>MDKDEAWKQVEILRRLGAKRIAYRSDDWRDLQEALKKGADILIVDATDKDEAWKQVEILRRLGAKEIAYRSDDWRDLQEALKKGADILIVDATDKDEAWKQVEILRRLGAKRIAYRSDDWRDLQEALKKGADILIVDATDKDEAWKQVEILRRLGAKEIAYRS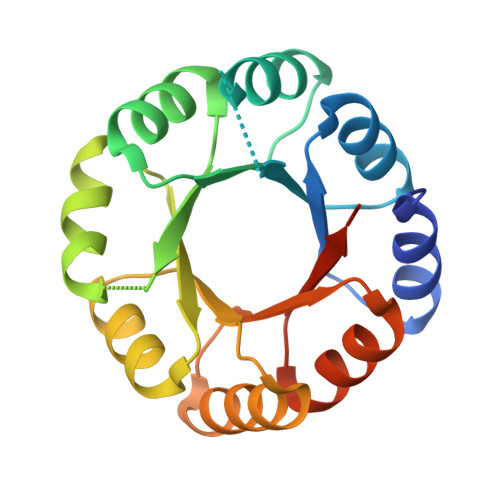DDWRDLQEALKKGADILIVDATGLEHHHHHH[2x]> MGSSHHHHHHSSGLVPRGSMSTSWSDRLQNAADMPANMDKHALKKYRREAYHRVFVNRSLAMEKIKCFGFDMDYTLAVYKSPEYESLGFELTVERLVSIGYPQELLSFAYDSTFPTRGLVFDTLYGNLLKVDAYGNLLVCAHGFNFIRGPETREQYPNKFIQRDDTERFYILNTLFNLPETYLLACLVDFFTNCPRYTSCETGFKDGDLFMSYRSMFQDVRDAVDWVHYKGSLKEKTVENLEKYVVKDGK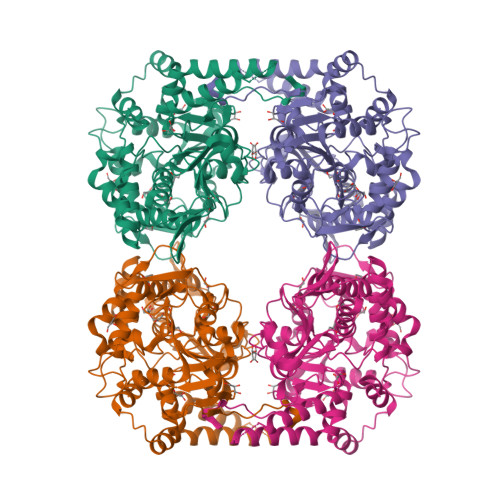LPLLLSRMKEVGKVFLATNSDYKYTDKIMTYLFDFPHGPKPGSSHRPWQSYFDLILVDARKPLFFGEGTVLRQVDTKTGKLKIGTYTGPLQHGIVYSGGSSDTICDLLGAKGKDILYIGDHIFGDILKSKKRQGWRTFLVIPEFAQELHVWTDKSSLFEELQSLDIFLAELYKHLDSSSNERPDISSIQRRIKKVTHDMDMCYGMMGSLFRSGSRQTLFASQVMRYADLYAASFINLLYYPFSYLFRAAHVLMPHESTVEHTHVDINEMESPLATRNRTSVDFKDTDYKRHQLTRSISEIKPPNL>[4x]GSIINETADDIVYRLTVIIDDRYE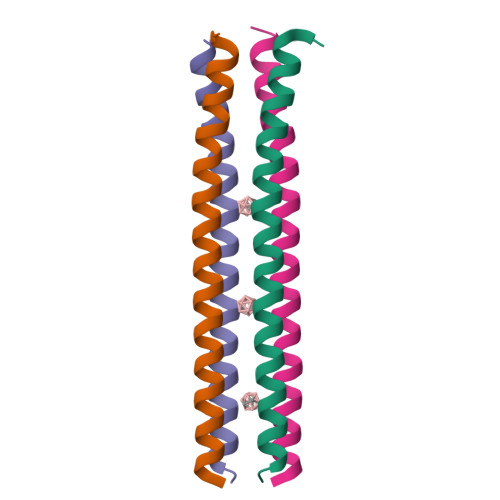SLKNLITLRADRLEMIINDNVSTILASI>[2x]CG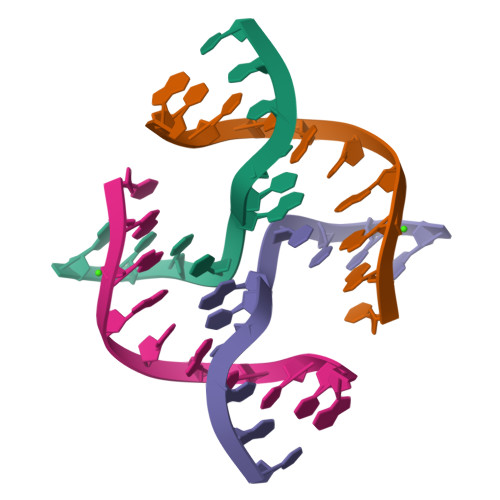GGTACCCG>[8x]AI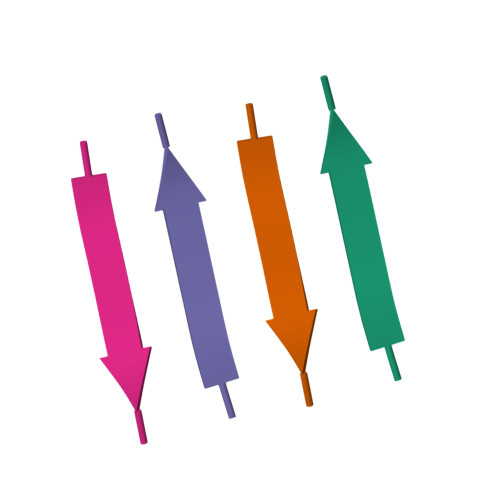LSST3-bromo-6-(4-nitro-1H-pyrazol-3-yl)pyrazolo[1,5-a]pyrimidin-2(1H)-one 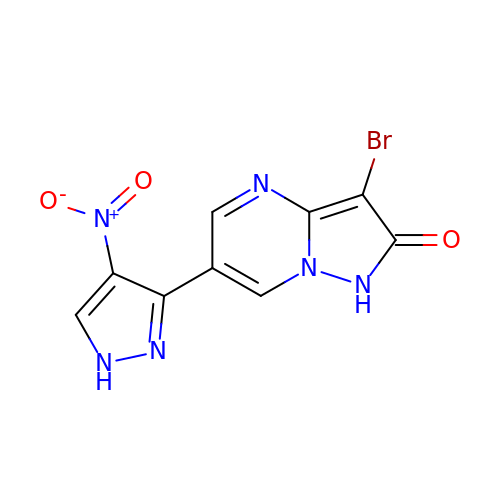| C9 H5 Br N6 O3 | GPUSMPJXAIFKFV-UHFFFAOYSA-N> MKIATITGVTKSPELQVTKAIGALILSSDVALSALTTEKISIYIERGNGSNVILANKVLLKDFILASTYGTENTQSDADNAMIALCELADEGSIYLADKESIKITLEDLISDKRYDLHGIEEPQQTNNLFFFEQKSVASEEFNKKIDVQGFDLAIMTVDDSV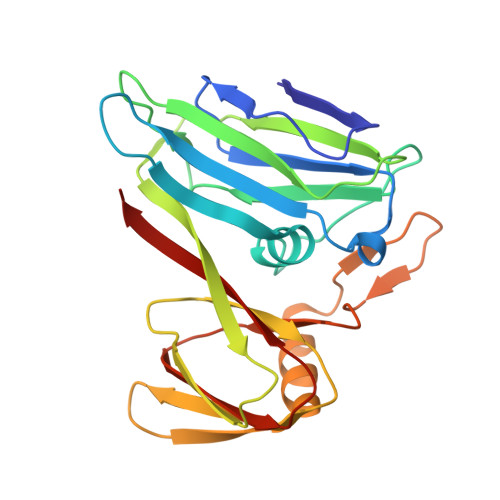SDLSYQYSNGQVVKYLPFELQTLSRDIDPIQAVLSDGKVVQGLTDRLTLPLVAVVGIEINKSQGSIINFVVRCLKTV4'-{6-methoxy-7-[2-(piperidin-1-yl)ethoxy]-1,2-dihydroindeno[1,2-c]pyrazol-3-yl}biphenyl-4-ol | C30 H31 N3 O3 | 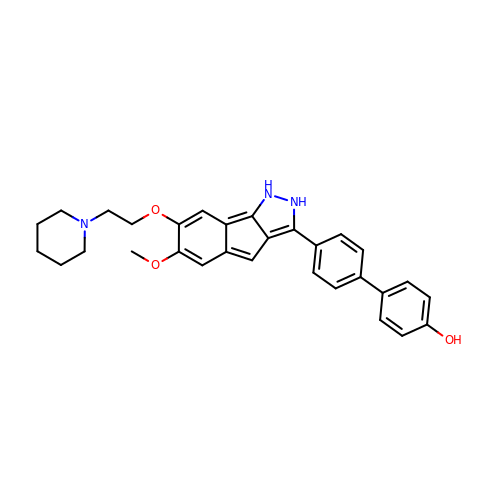DLRNUSDYANLOLU-UHFFFAOYSA-N>SGSVTAGMALAATDIPGLDASKLVSGVLAEQRLPVFARGLATAVSNSSDPNTATVPLMLTNHANGPVAGRYFYIQSMFYPDQNGNASQIATSYNATSEMYVRVSYAANPSIREWLPWQRCDIGGSFTKEADGELPGGVNLDSMVTSGWWSQSFTAQAASGANYPIVRAGLLHVYAASSNFIYQTYQAYDGESFYFRCRHSNTWFPWRRMWHGGDFNPSDYLLKSGFYWNALPGKPATFPPSAHNHDVGQLTSGILPLARGGVGSNTAAGARSTIGAGVPATASLGASGWWRDNDTGLIRQWGQVTCPADADASITFPIPFPTLCLGGYANQTSAFHPGTDASTGFRGATTTTAVIRNGYFAQAVLSWEAFGR[6x]

Morphologically and functionally, the R-type pyocins resemble the contractile tails of Myoviridae bacteriophages. Attachment of the fibers to the target cell surface causes structural changes in the baseplate that, in turn, trigger contraction of the external sheath, which drives the internal rigid tube through the host cell envelope. The killing mechanism of the pyocins is not specific to Pseudomonas, and their spectrum is fully determined by the fibers. We found that both R1 and R2 pyocin fiber fragments form a ~240 Å-long homotrimer that contains a rod-like and a shaft-like domain, two tandem knob domains, and the C-terminal lectin-like domain.

The iron-binding site has an octahedral geometry and is composed of six histidine residues—three symmetry-related copies of His561 and His563 in R1 and His562 and His564 in R2. A flat and nearly perfectly triangular density is located on the axis of the Knob2 of the R1 fiber, but no such feature is present in the R2. A similar triangular density is buried in the N-terminal part of the Shaft of the R2 fiber (residues Phe534-Tyr539), but there is no such “molecule” in the Shaft domain of the R1 fiber. In the R1 fiber, the grooves start at the threefold axis and extend radially outwards whereas in the R2 fiber the grooves are connected at the threefold axis, creating a “supercavity” at the tip of the fiber. The calcium cavity of R2 is located on the interface of two polypeptide chains and is much deeper than the sodium cavity of R1, which is formed by residues belonging to the same polypeptide chain. The coordination polyhedra of the calcium ions are mostly complete, with some water molecules replaced by ethylene glycol molecules that diffused into crystal during cryo protection. The calcium ion in the R2 structure takes its origins in the cell cytoplasm as the protein was never exposed to calcium containing salts during purification or crystallization. Notably, a chelating agent that is used during the purification procedure does not remove the calcium ion from the R2 fiber. In the structure of the R2 pyocin fiber, ethylene glycol molecules that mimic various parts of the LPS bind to the Knob2 and C-terminal domains. In the latter case, the interaction of the ethylene glycol molecule with the protein involves calcium ions, further supporting the role of calcium ions in binding to the LPS.N-(5-{[6-(5-methyl[1,2,4]triazolo[1,5-a]pyrimidin-7-yl)-2,6-diazaspiro[3.4]octan-2-yl]methyl}-1,3-thiazol-2-yl)acetamide 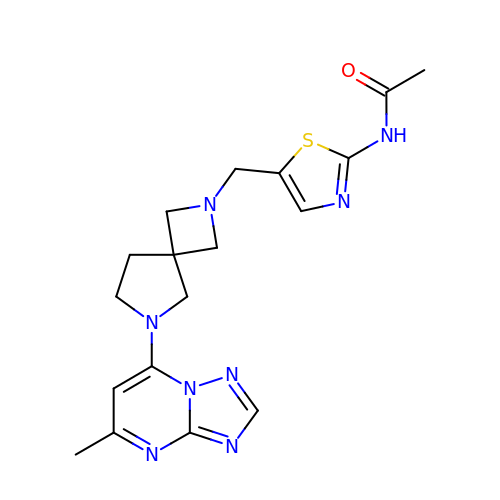| C18 H22 N8 O S | DSEWUBFXIVTHKH-UHFFFAOYSA-N> MQREEKQLEASLDALLSQVADLKNSLGSFICKLENEYGRLTWPSVLDSFALLSGQLNTLNKVLKHEKTPLFRNQVIIPLVLSPDRDEDLMRQTEGRVPVFSHEVVPDHLRTKPDPEVEEQEKQLTTDAARIGADAAQKQIQSLNKMCSNLLEKISKEERESESGGLRPNKQTFNPTDTNALVAAVAFGKGLSNWRPSGSSGPGQAGQPGAGTILAGTSGLQQVQMAGAPSQQQPMLSGVQMAQAGQPGKMPSGIK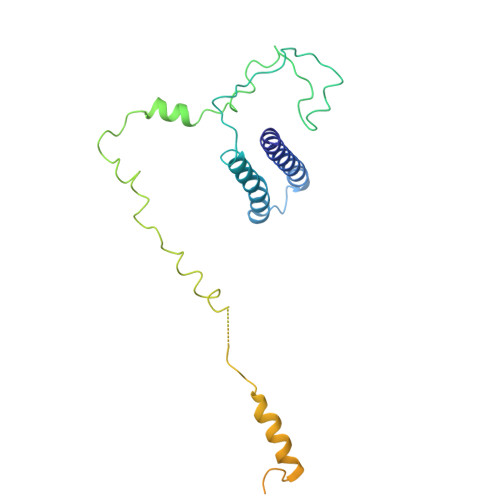TNIKSASMHPYQR>MAHHHHHHMKSIAQEHDCLLIDLDGTVF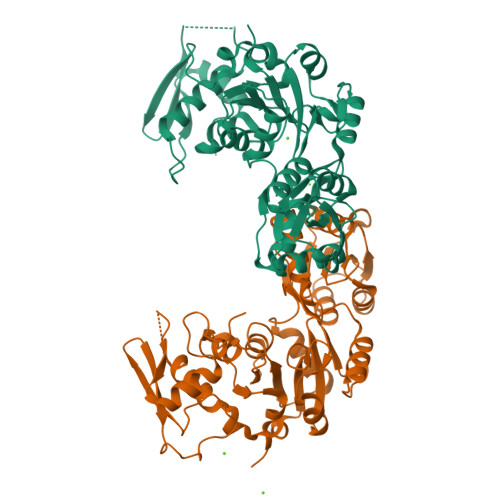CGRQPTGGAVQSLSQVRSRKLFVTNNASRSADEVAAHLCELGFTATGEDVVTSAQSAAHLLAGQLAPGARVLIVGTEALANEVAAVGLRPVRRFEDRPDAVVQGLSMTTGWSDLAEAALAIRAGALWVAANVDPTLPTERGLLPGNGSMVAALRTATGMDPRVAGKPAPALMTEAVARGDFRAALVVGDRLDTDIEGANAAGLPSLMVLTGVNSAWDAVYAEPVRRPTYIGHDLRSLHQDSKLLAVAPQPGWQIDVGGGAVTVCANGDVDDLEFIDDGLSIVRAVASAVWEARAADLHQRPLRIEAGDERARAALQRWSLMRSDHPVTSVGTQ[2x]Alginate is degraded by alginate lyases via a β-elimination mechanism to yield 4,5-unsaturated sugar at the non-reducing end. Persicobacter sp. CCB-QB2, an agarolytic bacterium isolated from seaweed (genus Ulva) in a coastal area of Malaysia9, was found to encode a PL7 alginate lyase, AlyQ, in its genome. Like many multidomain alginate lyases, AlyQ contains two additional carbohydrate-binding modules (CBMs) at its N terminus. AlyQ’s first domain moderately resembles family 16 CBM (CBM16), while the second domain belongs to family 32 CBM (CBM32).

In order to understand the relationship between these CBMs and the catalytic domain, we have characterized AlyQ’s activity and substrate binding, as well as solved the structure of a truncated version containing the CBM32 and catalytic domains. However, only AlyQBC successfully formed crystals, diffracting up to 2.2 Å in space group P41212 with one molecule in the asymmetric unit. In accordance to size-exclusion chromatography results, analysis with Pisa26 showed that all crystal contacts were not significant — AlyQBC exists as a monomer while domains B and C do not interact with one another. Residues E316–N321 in the region linking the two domains were disordered. A Ca2+ ion is found coordinated by the side chains of the strictly conserved D209 and T214, and the main chains of N206, N211, T214 and T307. W124 of YeCBM32, which when substituted with Ala resulted in only very weak affinity for the ligand polygalaturonic acid, is conserved in domain B as W303, and the region around this Trp, which is highly variable and involved in binding different sugars in CBM32 members, is also highly similar between AlyQ and YeCBM32. Moreover, an acetic acid molecule from the crystallisation buffer is found binding to the nearby R248, which may mimic the carboxyl group of an uronic acid. Subsites +1 to +3 are relatively well conserved between the two, and the three key residues for catalysis — Q436 neutralizing the substrate’s carboxyl group, H438 as a general base and Y541 as a general acid — were superposed well with A1-II’s Q189, H191 and Y284 to interact with the ligand, indicating AlyQ also employs a similar mechanism for alginate cleavage. A shift in AlyQ’s loop L1, however, is observed, which may represent the open conformation. Notably, if the GGMG ligand were to bind to AlyQ as it did to A1-II′, it would have crashed with AlyQ’s D446 and D447 at subsites +1 and −1 — D447 would especially repel the carboxyl group at subsite −1.

> MNHKVHMQYDIVAVTASAHDGNLPENTIDGNLSTRWSANGSGQYITFDLGSAKTVNQVKAAWYNGDSRTSGFSISLGSDPASLTEVYSGTSSGQTNALESYSFTATTARYIRITGFGNSSNTWNSITEVAIFHAGEEGDGNEEAPGTAQIPSDLMSNCNQWKITYPDGSEDKTLCGEANNEYWFVNEDKNAMVFRAPIRSNNGTTPNSSYVRSELRERKEDGSADIYWTTTGTHVVYVKQAITQLPIVKDHLVATQIHGDKSAGIDDAMVMRLEGNHLFASFNGGKLRSDLTIKTNYNLGTVHEVIFEVINGKHYLYYSEDGKLAEAYANGSAAAYLIKDGGNDYVMDLNYDQSYFKIGNYTQSNSEKEGSYTGDPNNYGEVVVYDYFVSHQHHHHHH>[2x]MSVDPMTYEAQFFGFTPQTCMLRIYIAFQDYLFEVMQAVEQVILKKLDGIPDCDISPVQIRKCTEKFLCFMKGHFDNLFSKMEQLFLQLILRIPSNILLPEDKCKETPYSEEDFQHLQKEIEQLQEKYKTELCTKQALLAELEEQKIVQAKLKQTLTFFDELHNVGRDHGTSDFRESLVSLVQNSRKLQNIRDNVEKESKRLKIS;>[2x]MTISRVKLLDTMVDTFLQKLVAAGSYQRFTDCYKCFYQLQPAMTQQIYDKFIAQLQTSIREEISDIKEEGNLEAVLNALDKIVEEGKVRKEPAWRPSGIPEK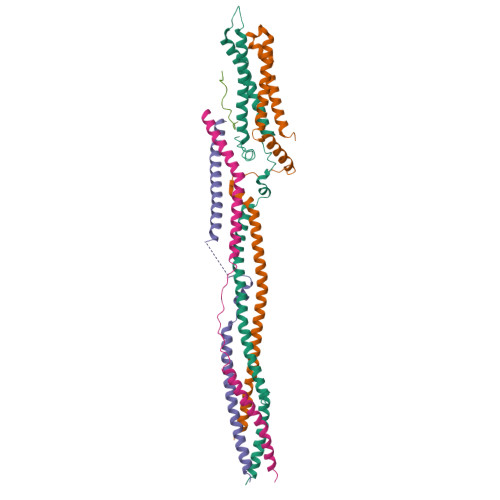DLHSVMAPYFLQQRDTLRRHVQKQEAENQQLADAVLAGRRQVEELQLQVQAQQQAWQALHREQRELVAVLREPE;>[2x]MGTLQKCFEDSNGKASDFSLEASVAEMKEYITKFSLERQTWDQLLLHYQQEAKEILSRGSTEAKITEVKVEPMTYLGSSQNEVLNTKPDYQKILQNQSKVFDCMELVMDELQGSVKQLQAFMDESTQCFQKVSVQLGKRSMQQLDPSPARKLLKLQLQNPPAIHGSGSGSCQHHHHHH;>MGQAWQEASDNCFMDSDIKVLEDQFDEIIVDIATKRKQYPRKILECVIKTIKAKQEILKQYHPVVHPLDLKYDPDPAPHMENLKCRGETVAKEISEAMKSLPALIEQGEGFSQVLR[2x];>GPLGSMAASGLDHLKNGYRRRFCRPSRARDINTEQGQNVLEILQDCFEEKSLANDFSTNSTKSVPNSTRKIKDTCI[2x]> DTMIPFDLSATKKNTME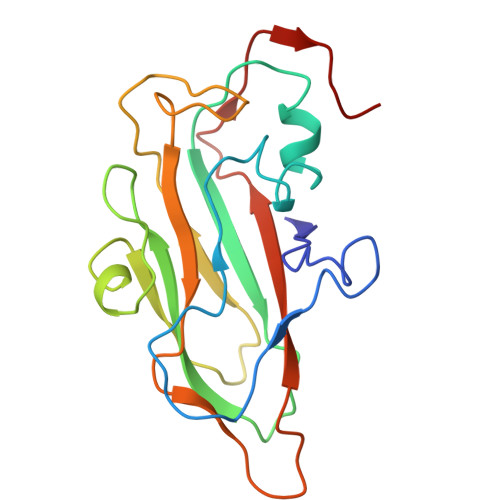MYRVRLSDKPHTDDPILCLSLSPASDPRLSHTMLGEILNYYTHWAGSLKFTFLFCGSMMATGKLLVSYAPPGADPPKKRKEAMLGTHVIWDIGLQSSCTMVVPWISNTTYRQTIDDSFTEGGYISVFYQTRIVVPLSTPREMDILGFVSACNDFSVRLLRDTTHI> MQTSARNQWFGTITARDHDDVQQHVDVLLADGKTRLKVAITAQSGARLGLDEGKEVLILLKAPWVGITQDEAVAQNADNQLPGIISHIERGAEQCEVLMALPDGQTLCATVPVNEATSLQQGQNVTAYFNADSVIIATLC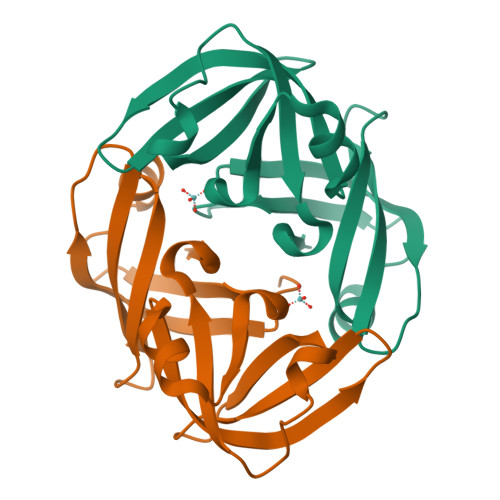;> MQTSARNQWFGTITARDHDDVQQHVDVLLADGKTRLKVAITAQSGARLGLDEGKEVLILLKAPWVGITQDEAVAQNADNQLPGIISHIERGAEQCEVLMALPDGQTLCATVPVNEATSLEQGQNVTAYFNADSVIIATLC>GSHHHHHHGGLNASYITPYVPMPCMINDTHFLLRGPFEASWAIKLEITDVTTLVVDTDNVANPTNISKCFANNQDERLLGFTMEWFLSGLEHDHHFTPQIICG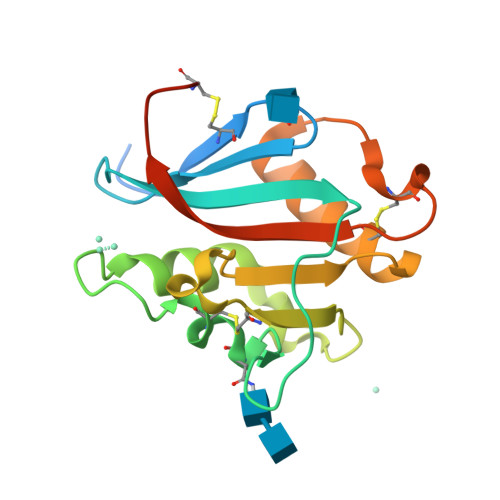NVSKGEVNAQVNITMEDHCSQVFLKMRRIFGVFKNPCTSHGKQNVLISVSNWTNQCSGNHLSSM[2x]> M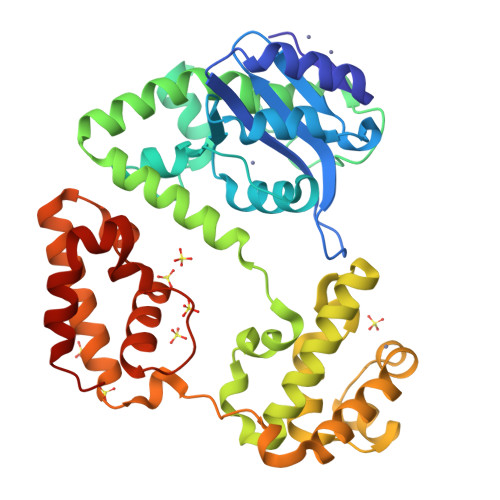NYQMITTDDALASLCEAVRAFPAIALDTEFVRTRTYYPQLGLIQLFDGEHLALIDPLGITDWSPLKAILRDPSITKFLHAGSEDLEVFLNVFGELPQPLIDTQILAAFCGRPMSWGFASMVEEYSGVTLDKSESRTDWLARPLTERQCEYAAADVWYLLPITAKLMVETEASGWLPAALDECRLMQMRRQEVVAPEDAWRDITNAWQLRTRQLACLQLLADWRLRKARERDLAVNFVVREEHLWSVARYMPGSLGELDSLGLSGSEIRFHGKTLLALVEKAQTLPEDALPQPMLNLMDMPGYRKAFKAIKSLITDVSETHKISAELLASRRQINQLLNWHWKLKPQNNLPELISGWRGELMAEALHNLLQEYPQ>[2x]MSSVT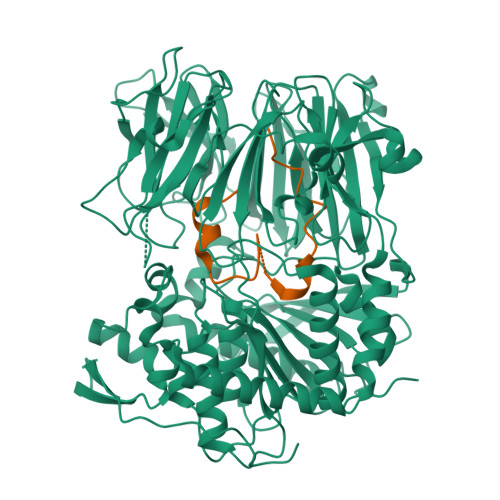WAPGNYPSTRRSDHVDTYQSASKGEVPVPDPYQWLEESTDEVDKWTTAQADLAQSYLDQNADIQKLAEKFRASRNYAKFSAPTLLDDGHWYWFYNRGLQSQSVLYRSKEPALPDFSKGDDNVGDVFFDPNVLAADGSAGMVLCKFSPDGKFFAYAVSHLGGDYSTIYVRSTSSPLSQASVAQGVDGRLSDEVKWFKFSTIIWTKDSKGFLYQRYPARERHEGTRSDRNAMMCYHKVGTTQEEDIIVYQDNEHPEWIYGADTSEDGKYLYLYQFKDTSKKNLLWVAELDEDGVKSGIHWRKVVNEYAADYNIITNHGSLVYIKTNLNAPQYKVITIDLSKDEPEIRDFIPEEKDAKLAQVNCANEEYFVAIYKRNVKDEIYLYSKAGVQLTRLAPDFVGAASIANRQKQTHFFLTLSGFNTPGTIARYDFTAPETQRFSILRTTKVNELDPDDFESTQVWYESKDGTKIPMFIVRHKSTKFDGTAAAIQYGYGGFATSADPFFSPIILTFLQTYGAIFAVPSIRGGGEFGEEWHKGGRRETKVNTFDDFIAAAQFLVKNKYAAPGKVAINGASNGGLLVMGSIVRAPEGTFGAAVPEGGVADLLKFHKFTGGQAWISEYGNPSIPEEFDYIYPLSPVHNVRTDKVMPATLITVNIGDGRVVPMHSFKFIATLQHNVPQNPHPLLIKIDKSWLGAGMGKPTDKNVKDAADKWGFIARALGLELKTVEMFDTNATRLPIWGIGCNPWTAEHVDQTLASGNDIC;>MFDTNATRLPIWGIGCNPWTAEHVDQTLASGNDIC[2x]> GAQVSSQKVGAHENSNRAYGGSTINYTTINYYRDSASNAASKQDFAQDPSKFTEPIKDVLIK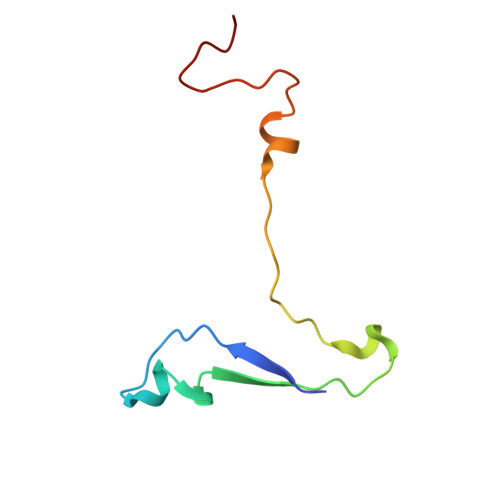TAPTLN>[2x]PQPPADEQPEPRTRRR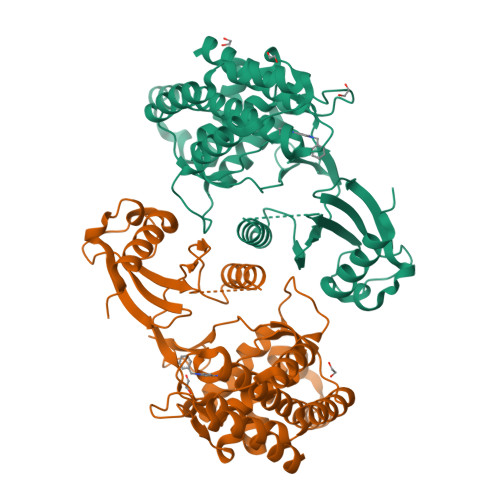AYLWCKEFLPGAWRGLREDEFHISVIRGGLSNMLFQCSLPDTTATLGDEPRKVLLRLYGAILQMRSCNKEGSEQAQKENEFQGAEAMVLESVMFAILAERSLGPKLYGIFPQGRLEQFIPSRRLDTEELSLPDISAEIAEKMATFHGMKMPFNKEPKWLFGTMEKYLKEVLRIKFTEESRIKKLHKLLSYNLPLELENLRSLLESTPSPVVFCHNDCQEGNILLLEGRENSEKQKLMLIDFEYSSYNYRGFDIGNHFCEWMYDYSYEKYPFFRANIRKYPTKKQQLHFISSYLPAFQNDFENLSTEEKSIIKEEMLLEVNRFALASHFLWGLWSIVQAKISSIEFGYMDYAQARFDAYFHQKRKLGV> MHHHHHHENTSVQNKETVRNCPFDYAHELEFDPQLRQLLTEEPVSRIRMAYGEGEAWLVTRYEDVRTVTTDRRFSRSAVLGRDFPRMTPEPIVQAESINLMDPPASSRLRGLVAKSFTPRRVEQMRGGTQRVVDRLLDEMEEEGSPADFVARVSAPLPLITICEALDIPEADRPWLRAHAMTMMNVGAAGKQDAVRAKAELRGYFQELTADRRRSPGEDLISTLATARDGDELLDDDELAVMAMVLLITGQDTTTYQLGNIAYTLLTRPDLLRSLRAEPQRLPRTLEELLRHIPFRKGVGIPRIALEDVELSGVLIKAGDVVHVSYLTANRDSAKFDRPDELDPDRPTIPHMTFGWGAHHCLGAPLATMEL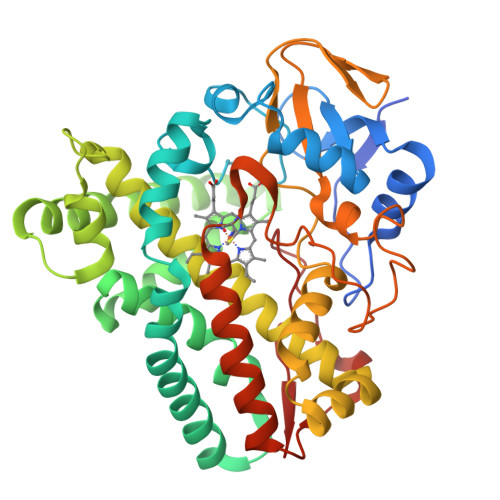EVAFSTLLTRFPALRLDVPPEDVSWNTTSIWRYPLALPVTW> AIDLCGMSQDELNECKPAVSKENPT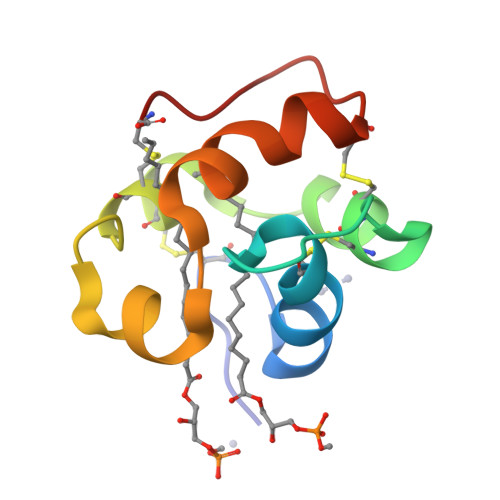SPSQPCCTALQHADFACLCGYKNSPWLGSFGVDPELASALPKQCGLANAPTC> GSHMGAGYNSEDEYEAAAARIEAMDPATVEQQEHWFEKALRD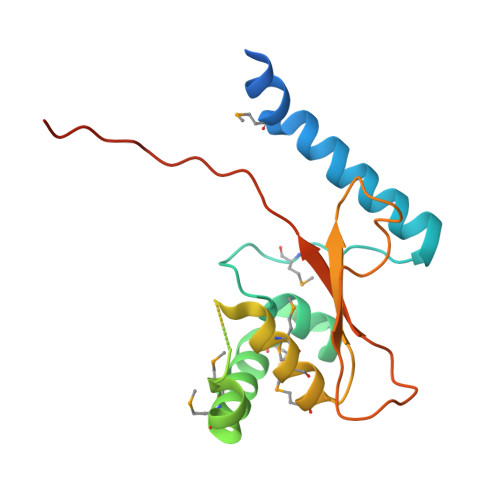KKGFIIKQMKEDGACLFRAVADQVYGDQDMHEVVRKHCMDYLMKNADYFSNYVTEDFTTYINRKRKNNCHGNHIEMQAMAEMYNRPVEVYQYSTGTSAVEPINTFHGIHQNEDEPIRVSYHRNIHYNSVVNPNKATIGVGLG Griselimycins (GMs) are such promising anti-TB antibiotics that bind and inhibit the mycobacterial DNA polymerase III sliding clamp (DnaN). Although the co-crystal of msDnaN and MP A could not be obtained after intensive attempts, DnaN of E. coli (ecDnaN) was overproduced in E. coli and co-crystallized with MP A, GM and cyclohexyl-GM (CGM). Despite sharing only 29 % sequence identity with msDnaN, the binding pocket of ecDNA shows a sufficient degree of conservation. The binding pocket can be divided into a larger (subsite 1) and a smaller cavity (subsite 2) and as has been shown previously for GM and mycobacterial DnaN, all compounds occupy both subsites of the binding pocket.

The crystal structures were solved at resolutions of 2.12 Å (MP A), 1.65 Å (GM) and 1.50 Å (CGM). MP A was found to bind in the same mode to ecDnaN as GM or CGM. All three substances form hydrogen bonds to only 2 – 3 protein residues, but the additional oxygen in the N-terminal α-keto butyrate residue of MP A provides a second hydrogen bond acceptor for Arg365, which is also conserved in mycobacterial DnaN. The compounds bind mainly via van der Waals interactions with interfaces ranging from 550 Å2 for GM to 590 Å2 for CGM to 600 Å2 for MP A. Compared to available structures of uncomplexed DnaN, only a few residues undergo significant conformational changes upon binding of the compounds - most notably Met362, which has been described to function as a gate between the subsites. The linear, N-terminal part of the ligands in subsite 2 superimposes almost perfectly, while MP A seems to be tilted slightly (approximately 7-10 ° compared to GM/CGM) away from the protein in the region around Pro8. This tilting can be attributed to the longer 5-methyl-l-norleucine residue of MP A at position 6, whereas leucine is present at the same position in GM and CGM. The comparison with the previously published mycobacterial GM/DnaN complexes shows that whereas the N-terminal parts of the ligands in subsite 2 superimpose very well, there is higher variance on the opposite side of the molecules around Pro8. In complex with M. tuberculosis DnaN, the tilt of GM away from the protein is less pronounced, instead the macrocycle seems to be tilted approximately 7° towards positon 7 in comparison to the msDnaN complex. Although differences in crystal packing make a direct comparison of the binding strength difficult, the linear part of the ligands (1-3) and the residues adjacent to the bifurcation seem to be bound tighter/show less flexibility than the opposing residues (6-9) in all structures of DnaN/GM complexes. The highest affinity to M. smegmatis DnaN (msDnaN) was observed for GM with KD = 6.5 ± 5.9 nM. Interestingly, GM manifests a slightly stronger DnaN binding affinity than the MPs but is less active than MPs against mycobacteria.

> GGRMKFTVEREHLLKPLQQVSGPLGGRPTLPILGNLLLQVADGTLSLTGTDLEMEMVARVALVQPHEPGATTVPARKFFDICRGLPEGAEIAVQLEGERMLVRSGRSRFSLSTLPAADFPNLDDWQSEVEFTLPQATMKRLIEATQFSMAHQDVRYYLNGMLFETEGEELRTVATDGHRLAVCSMPIGQSLPSHSVIVPRKGVIELMRMLDGGDNPLRVQIGSNNIRAHVGDFIFTSKLVDGRFPDYRRVLPKNPDKHLEAGCDLLKQAFARAAILSNEKFRGVRLYVSENQLKITANNPEQEEAEEILDVTYSGAEMEIGFNVSYVLDVLNALKCENVRMMLTDSVSSVQIEDAASQSAAYVVMPMRL;> XVPTLPLVPXG> YATLLDLDPKGKRVLVRVDYNVPVQDGKVQDETRILESLPTLRHLLAGGASLVLLSHLGRPKGPDPRYSLAPVGEALRAHLPEARFAPFPPGSEEAR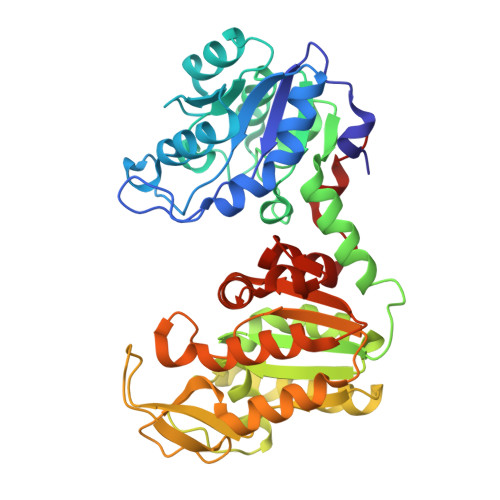REAEALRPGEVLLLENVRFEPGEEKNDPELSARYARLGEAFVLDAFGSAHRAHASVVGVARLLPAYAGFLMEKEVRALSRLLKDPERPYAVVLGGAKVSDKIGVIESLLPRIDRLLIGGAMAFTFLKALGGEVGRSLVEEDRLDLAKDLLGRAEALGVRVYLPEDVVAAERIEAGVETRVFPARAIPVPYMGLDIGPKTREAFARALEGARTVFWNGPMGVFEVPPFDEGTLAVGQAIAALEGAFTVVGGGDSVAAVNRLGLKERFGHVSTGGGASLEFLEKGTLPGLEVLEG8-(naphthalen-1-yl)quinoline-2-carboxylic acid | C20 H13 N O2 | 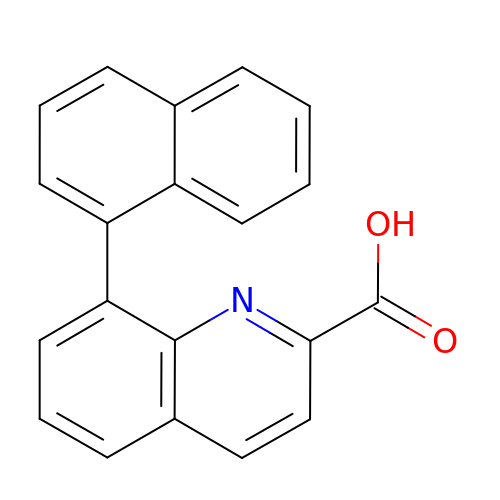QMAYJELNBDAEMC-UHFFFAOYSA-N>[2x]NMSEVINFDQIFEGAIEPGKEPKRLFKEVYEGAITATSYAEILLSRAIEKYGPDHPVGYPDTAYFL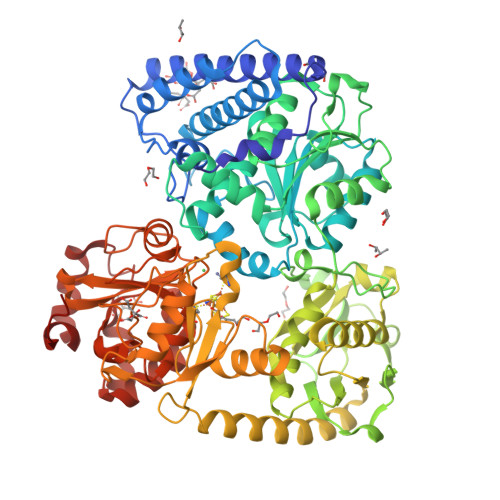PVIRAFSGEEVRTLKDMVPILNRMRAQIKSELTFENARLAGEATWYAAEIIEALRYLKHTPENPIVVPPWTGFIGDPVVRQYGIKMVDWTIPGEAIIIGRAKDSKAAKKIVDDLMGKGLMLFLCDEIIEQLLEENVKLGVDYIAYPLGNFTQVVHAANYALRAGLMFGGIAPGLRDAHRDYQRRRVLAFVLYLGEHDMVKTAAAMGAIFTGFPVITDQPLPEDKQIKDWFISEPDYDKIVQTALEVRGIKITSIDIDLPINFGPAFEGESIRKGDMHVEFGGGKTPSFELVRMVGPDEIEDGKVEVIGPDIDSVEPGGRLPIGIVVDIYGRKMQEDFEPVLERRIHYFTNYGEGFWHTAQRDLTWVRISKEAFAKGARLKHLGQLLYAKFKQEFPSIVDRVQVTIYTDEQKVLELREIARKKYAERDARLRELSDEAVDTYYSCLLCQSFAPTHVCIVSPERVGLCGAISWLDAKAAYEINPNGPNQPIPKEGLIDPVKGQWESFNEYIYKNSQRTIERMNLYTIMEYPMTSCGCFEAIMAYLPELNGFMIVNREHSGMTPIGMTFSTLAGMVGGGTQTPGFMGIGKSYIGSRKFVKADGGLARVVWMPKDLKEQLRSIIEERAEEEGLGRDFIDKIADETVGTTVDEVLPFLEEKGHPALSMEPLL> GSSHSSANEDMPVERILEAELAVEPKTETYVEANMGLNPSSPNDPVTNICQ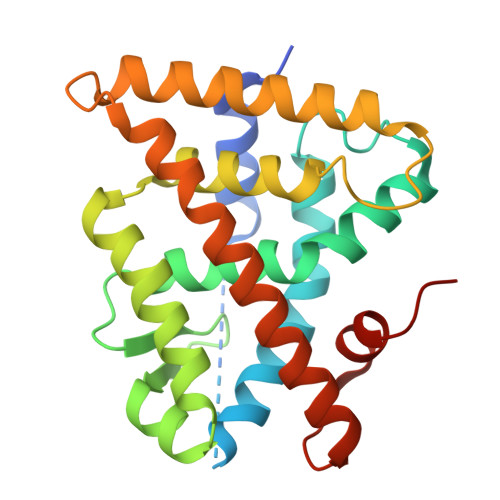AADKQLFTLVEWAKRIPHFSELPLDDQVILLRAGWNELLIASFSHRSIAVKDGILLATGLHVHRNSAHSAGVGAIFDRVLTELVSKMRDMQMDKTELGCLRAIVLFNPDSKGLSNPAEVEALREKVYASLEAYCKHKYPEQPGRFAKLLLRLPALRSIGLKCLEHLFFFKLIGDTPIDTFLMEMLEAPHQMT> AQTVPYGIPLIKADKVQAQGYKGANVKVGIIDTGIASSHTDLKVVGGASFVSGESYNTDGNGHGTHVAGTVAALDNTTGVLGVAPNVSLYAIKVLNSSGSGSYSAIVSGIEWATQNGLDVINMSLGGPSGSTALKQAVDKAYASGIVVVAAAGNSGNSGSQNTIGYPAKYDSVIAVGAVDSNKNRASFSSVGSELEVMAPGVSVYSTYPSNTYTSLNGTS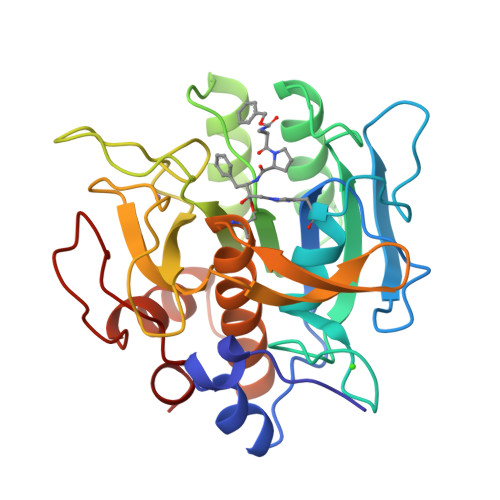MASPHVAGAAALILSKYPTLSASQVRNRLSSTATNLGDSFYYGKGLINVEAAAQ> GDPIADMIDQTVNNQVNRSLTALQVLPTAANTEASSHRLGTGVVPALQAAETGASSNASDKNLIETRCVLNHHSTQETAIGNFFSRAGLVSIITMPTTGTQNTDGYVNWDIDLMGYAQLRRKCELFTYMRFDAEFTFVVAKPNGELVPQLLQYMYVPPGAPKPTSRDSFAWQTATNPSVFVKMTDPPAQVSVPFMSPASAYQWFYDGYPTFGEHLQANDLDYGQCPNNMMGTFSIRTVGIEKSPHSITLRVYMRIKHVRAWIPRPLRNQPYLFKTNPNYKGNDIKCTSTSRDKITTL;> MGSQVSTQRSGSHENSNSASEGSTINYTTINYYKDAYAASAGRQDMSQDPKKFTDPVMDVIHEMAPPLKSPSAEACGYSDRVAQLTIGNSTITTQEAANIVIAYGEWPEYCPDTDATAVDKPTRPDVSVNRFFTLDTKSWAKDSKGWYWKFPDVLTEVGVFGQNAQFHYLYRSGFCVHVQCNASKFHQGALLVAVLPEYVLGTIAGGTGNENSHPPYATTQPGQVGAVLTHPYVLDAGIPLSQLTVCPHQWINLRTNNCATIIVPYMNTVPFDSALNHCNFGLLVIPVVPLDFNTGATSEIPITVTIAPMCAEFAGLRQAVKQ;> GIPTELKPGTNQFLTTDDGVSAPILPGFHPTPPIHIPGEVHNLLEICRVETILEVNNLKTNETTPMQRLCFPVSVQSKTGELCAAFRADPGRDGPWQSTILGQLCRYYTQWSGSLEVTFMFAGSFMATGKMLIAYTPPGGNVPADRITAMLGTHVIWDFGLQSSVTLVVPWISNTHYRAHARAGYFDYYTTGIITIWYQTNYVVPIGAPTTAYIVALAAAQDNFTMKLCKDTEDIEQTANIQ

Enterovirus 71 (EV71) and coxsackievirus A16 (CVA16) are subgroup A human enteroviruses (HEVA), small, nonenveloped single-stranded RNA (ssRNA) viruses whose protective capsid mediates cell entry and humoral immune responses. The external portion of the icosahedral capsid comprises 60 copies of viral proteins VP1, -2, and -3 arranged with pseudo T=3 symmetry, while their N-terminal extensions and 60 copies of VP4 line the interior, surrounding the RNA genome. There is a “canyon” (a depression encircling the 5-fold axes) on the surface of enteroviruses that often harbors the receptor binding site, and there is a fatty acid binding site below the canyon base, within the hydrophobic β-barrel core of VP1. Here, we remedy this with high resolution X-ray structures of both mature and natural empty CVA16 particles and also of empty recombinant viruslike particles of CVA16 produced in insect cells, a potential vaccine antigen.

Natural empty particles (without RNA) are often also formed, in which the final RNA-mediated coat protein cleavage (between VP4 and VP2) is not made. The sedimentation coefficients and λ260/λ280 absorbance ratios were ∼160S and 1.67 for the mature virus, and ∼80S and 0.64 for the empty particle, indicating that the latter does not contain RNA, and SDS-PAGE showed that VP0 is not cleaved into VP4 and VP2 in the empty particle. Diffraction data for inactivated CVA16 empty and full virus particles to 2.7- and 2.65-Å resolution, respectively, were collected at room temperature in situ. The natural empty particle is not expanded. The natural empty particle contains proteins VP0, VP1, and VP3. Residues lining the inner surface of the particle are more flexible (with higher B factors) and some residues are essentially disordered, and thus, residues 9 to 18 and 39 to 42 in VP1 and 1 to 11 and 62 to 80 in VP0 (corresponding to 1 to 11 and 61 to 69 of VP4 and 1 to 9 of VP2 in the mature particle) are not defined in the electron density map. The overall structure is otherwise essentially indistinguishable from that of the mature virus (RMSD of 0.3 Å for 813 Cα atoms), and the pocket factor binding site is fully occupied by a moiety that again resembles sphingosine. However, the inner surface of the empty CVA16 particle is much more ordered than the expanded EV71 empty particle, where the entire 69 residues of VP4 and residues 1 to 72 of VP1 are invisible. The EV71 natural empty particles used in our earlier structural studies (produced by two independent companies) and those from a different strain used in another structural analysis were all in an expanded conformation, while using identical methodology, those for CVA16 described here are not (although we have observed an expanded CVA16 intermediate [135S] particle).>MSLTITVLQGGNVLDLERGVLLEHHHVVIDGERIVEVTDRPVDLPNAQAIDVRGKTVMPGFIDCHVHVLASNANLGVNATQPNILAAIRSLPILDAMLSRGFTSVRDAGGADWSLMQAVETGLVSGPRIFPSGKALSQTGGHGDFRPRGDL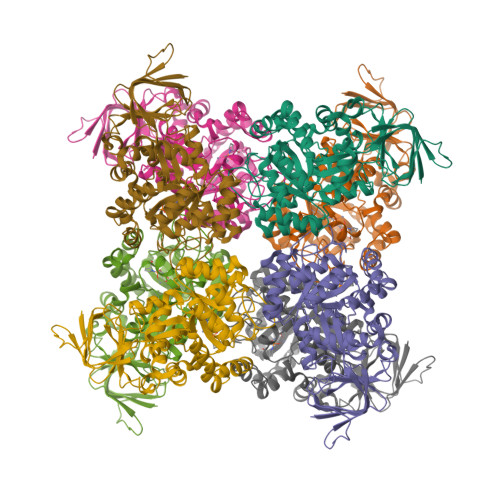LEPCSCCFRTGAIARVVDGVEGVRLAVREEIQKGATQIKIMASGGVASPTDPIANTQYSEDEIRAIVDEAEAANTYVMAHAYTGRAIARAVRCGVRTIEHGNLVDEAAAKLMHEHGAFVVPTLVTYDALAKHGAEFGMPPESVAKVASVQQKGRESLEIYANAGVKMGFGSDLLGEMHAFQSGEFRIRAEVLGNLEALRSATTVAAEIVNMQGQLGVIAVGAIADLVVLDGNPLEDIGVVADEGARVEYVLQRGTLVKRQAAGREGHHHHHH[16x]>MKTSKTKTPKSVLIAGPCVIESLENLRSIATKLQPLANNERLDFYFKASFDKANRTSLESYRGPGLEKGLEMLQTIKEEFGYKILTDVHESYQASVAAKVADILQIPAFLCRQTDLIVEVSQTNAIVNIKKGQFMNPKDMQYSVLKALKTRDKSIQSPTYETALKNGVWLCERGSSFGYGNLVVDMRSLKIMREFAPVIFDATASVQMPGGA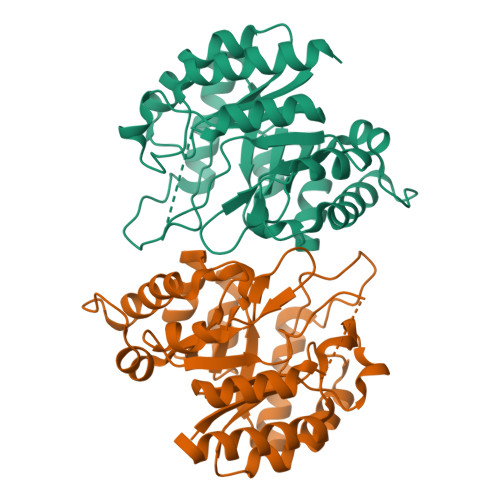NGKSSGDSSFAPILARAAAAVGIDGLFAETHVDPKNALSDGANMLKPDELEQLVTDMLKIQNLF[2x]>[2x]GAKSRDAEFVPFPERVSIEEYISRQLPEISSVAVPVAAETGGELTVMGLPYVQVCGTGDTQGYRVVGYTTVAPSMSFERLEKLVTENKPDWAVAVQVDKQIDRDATRGIQLIDNYGG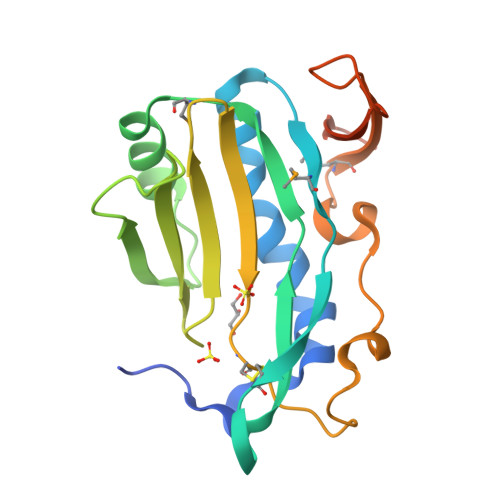LVEFKFSEDSIAVRSRSACLPTNKPLDDPGQFVLPSVEEAFPGMHVTISDNTNPDLHPVPTLTTGAHVTPQSGTQSGTQSGS>[2x]DLADRFAELERRYDARLGVYVPATGTTAAIEYRADERFAFCSTFKAPLVAAVLHQNPLTHLDKLITYTSDDIRSISPVAQQHVQTGMTIGQLCDAAIRYSDGTAANLLLADLGGPGGGTAAFTGYLRSLGDTVSRLDAEESELNRDPPGDERDTTTPHAIALVLQQLVL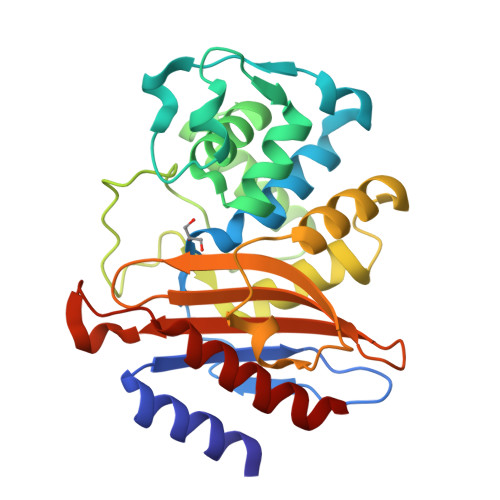GNALPPDKRALLTDWMARNTTGAKRIRAGFPADWKVIDKTGTGDYGRANDIAVVWSPTGVPYVVAVMSDRAGGGYDAEPREALLAEAATCVAGVLA> PLSEIPTDDNPNMSMAEMLRRDEGLRLKVYWDTEGYPTIGIGHLIMKQPVRDMAQINKVLSKQVGREITGNPGSITMEEATTLFERDLADMQRDIKSHSKVGPVWQAVNRSRQMALENMAFQMGVGGVAKFNTMLTAMLAGDWEKAYKAGRDSLWYQQTKGRASRVTMIILTGNLESYGVE;> GYDKDLCEWSMTADQTEVETQIEADIMNIVKRDRPEMKAEVQKQLKSGGVMQYNYVLYCDKNFNNKNIIAEVVGE

Here, we describe the structure and function of gp61.3 and show that gp61.3 inhibits the lysozyme activity of gp5 but not that of T4L. In 2002, we determined the crystal structure of gp5 that showed that gp5 consists of three domains: an N-terminal OB-fold (Oligonucleotide/Oligosaccharide-Binding fold, gp5OB-fold, residues 1–129), a lysozyme domain (gp5Lys, residues 174–339), and a needle-like C-terminal β-helical domain (gp5β, residues 389–575). We hypothesized that the mature form of Spackle/gp61.3 (residues 23–97) functions in the periplasm to selectively inhibit the activity of gp5, possibly by direct interaction. Combining all our results with previous work on gene sp and 5 mutants, we propose that the main function of the Spackle protein gp61.3 is to inhibit “free” copies of gp5 that are not incorporated into the virion during T4 particle assembly and thus can escape into the periplasm.

To understand the interaction between gp61.3 and gp5Lys, we crystallized the complex of gp61.3 and gp5Lys obtained (Lane 5), solved its crystal structure by Molecular Replacement and refined it to a resolution of 1.15 Å. The complex consists of one molecule of gp61.3 and one molecule of gp5Lys. The crystal structure contains a fragment of a poly (ethylene glycol) methyl ether molecule (a chemical that was used in the crystallization), four ethylene glycol molecules, three sodium ions, one chloride ion and 382 water molecules. The interface between gp5 and gp61.3 contains 10 hydrogen bonds and 8 salt bridges. The buried surface area is 1733.1 Å2. The two jaw-like subdomains of gp5Lys are further away from each in the gp61.3-gp5 complex compared to that in the gp5 trimer. Thus, upon interaction with gp61.3, gp5Lys becomes “frozen” in an open jaw-like state. In the gp61.3-gp5Lys complex, gp61.3 forms a wall at one of the cleft’s exits, which likely abolishes the endoglycosidase activity of gp5Lys or turns it into an exoglycosidase with a much-reduced turnover rate of polymeric substrate (the peptidoglycan). Therefore, gp61.3 inhibits gp5Lys allosterically by stabilizing one conformation in the gp5Lys catalytic cycle, thus breaking it. Gly322 fits against the C-terminus of helix 5 of gp61.3 (which forms the C-terminus of the protein) so that it leaves no space for a side chain.> ETG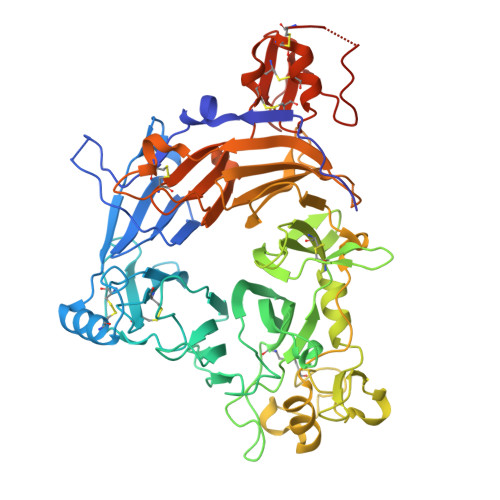GFPEDSEPISISHGNYTKQYPVFVGHKPGRNTTQRHRLDIQMIMIMNRTLYVAARDHIYTVDIDTSHTEEIYCSKKLTWKSRQADVDTCRMKGKHKDECHNFIKVLLKKNDDTLFVCGTNAFNPSCRNYRVDTLETFGDEFSGMARCPYDAKHANIALFADGKLYSATVTDFLAIDAVIYRSLGDSPTLRTVKHDSKWLKEPYFVQAVDYGDYIYFFFREIAVEYNTMGKVVFPRVAQVCKNDMGGSQRVLEKQWTSFLKARLNCSVPGDSHFYFNILQAVTDVIRINGRDVVLATFSTPYNSIPGSAVCAYDMLDIANVFTGRFKEQKSPDSTWTPVPDERVPKPRPGCCAGSSSLEKYATSNEFPDDTLNFIKTHPLMDEAVPSIINRPWFLRTMVRYRLTKIAVDNAAGPYQNHTVVFLGSEKGIILKFLARIGSSGFLNGSLFLEEMNVYNPEKCSYDGVEDKRIMGMQLDRASGSLYVAFSTCVIKVPLGRCERHGKCKKTCIASRDPYCGWVRESGSCAHLSPLSRLTFEQDIERGNTDGLGDCHNSGTKHHHHHH>[10x]MYQHQSTEAASHLEATPYFREDPRLTGFRHRFDTVDGVRLHFVEGGRADGETIVLLAGFPESWYAWRRVMPLLADEFRIVAPDLPGQGDSDRPLVGYDTQTVAATLARLLERQNIARFYLAAH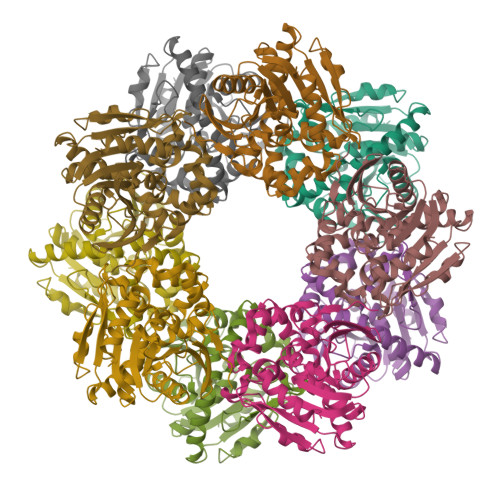DVGAWVAYPFAAMYPESVKRLALLDAGIPGVTLPAALPIEPGNAWRTWHFAFHTVADLPETLIAGKEREYLDWFLRRKAANPESFSDADVDEYLRVFTRDGGLRAGLAFYRAVSESSAQNRKLQALGKLKMPVLAVSADQGSIPDMAGPLEHVAEEVTAATIAYSGHFIPEEQPQALARELRDFFR> GSDSVKIIRLVKNREPLGATIKKDEQTGAIIVARIMRGGAADRSGLIHVGDELREVNGIPVEDKRPEEIIQILAQSQGAITFKIIP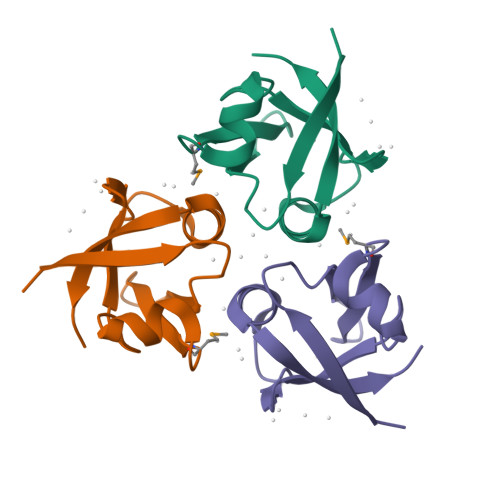GSKEETP>[6x]MSKMRFFALQELSNRKPLEITTPSNKLSDYYASHVFDRKKMQEYLPKEAYKAVVDATEKGTPISREMADLIANGMKSWAKSLNVTHYTHWFQPLTDGTAEKHDGFIEFGEDGEVIERFSGKLLIQQEPDASSFPNGGIRNTFEARGYTAWDGSSPAFVVDTTLCIPTIFISYTGEALDYKTPLLKALAAVDKAATEVCQLFDKNITRVFTNLGWEQEYFLVDTSLYNARPDLRLTGRTLMGHSSAKDQQLEDHYFGSIPPRVTAFMKELEIECHKLGIPVKTRHNEVAPNQFELAPIFENCNLANDHNQLVMDLMKRIARKHHFAVLFHEKPYNGVNGSGKHNNWSLCTDTGINLFAPGKNPKGNMLFLTFLVNVL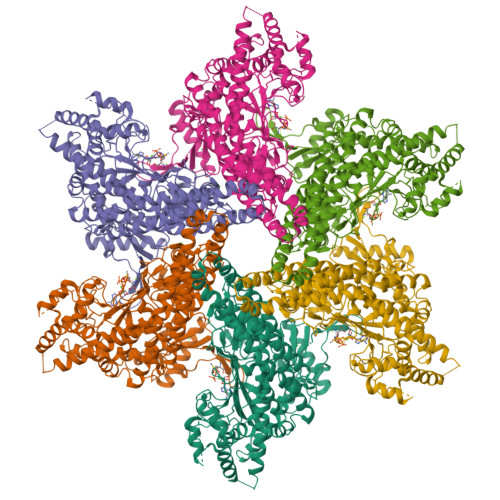MMVHKNQDLLRASIMSAGNSHRLGANEAPPAILSIFLGSQLSATLDEIVRQVTNSKMTPEEKTTLKLGIGRIPEILLDTTDRNRTSPFAFTGNRFEFRAAGSSANCAAAMIAINAAMANQLNEFKASVDKLMEEGIGKDEAIFRILKENIIASELIRFEGDGYSEEWKQEAARRGLTNICHVPEALMHYMDNQSRAVLIGERIFNETELACRLEVELEKYTMKVQIESRVLGDLAINHIVPIAVSYQNRLLENLCRMKEIFSEEEYEVMSADRKELIKEISHRVSAIKVLVRDMTEARKVANHKENFKEKAFAYEETVRPYLESIRDHIDHLEMEIDDEIWPLPKYRELLFTK> SKSTTLFSRHTKAIVWGMQTRAVQGMLDFDYVCSRDEPSVAAMVYPFTGDHKQKFYWGHKEILIPVFKNMADAMRKHPEVDVLINFASLRSAYDSTMETMNYAQIRTIAIIAEGIPEALTRKLIKKADQKGVTIIGPATVGGIK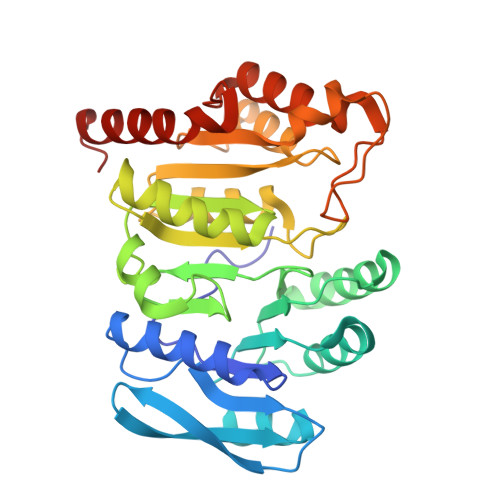PGCFKIGNTGGMLDNILASKLYRPGSVAYVSRSGGMSNELNNIISRTTDGVYEGVAIGGDRYPGSTFMDHVLRYQDTPGVKMIVVLGEIGGTEEYKICRGIKEGRLTKPIVCWCIGTCATMFSSEVQFGHAGACANQASETAVAKNQALKEAGVFVPRSFDELGEIIQSVYEDLVANGVI2-{[2-(4-chlorophenyl)-2-oxoethyl]sulfanyl}benzoic acid | C15 H11 Cl O3 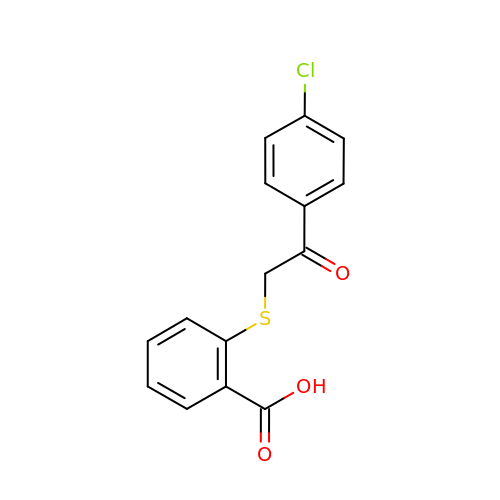S | SWPTTWQFPBNDMV-UHFFFAOYSA-N> MFENITTAPADPILGLADLFRADERPGKINLGIGVYKDETGKTPVLTSVKKAEQYLLENETTKNYLGIDGIPEFGRCTQELLFGKGSALINDKRARTAQTPGGTGALRVAADFLAKNTSVKRVWVSNPSWPNHKSVFNSAGLEVREYAYYDAENHTLDFDALINSLNEAQAGDVVLFHGCCHNPTGIDPTLEQWQTLAQLSVEKGWLPLFDFAYQGFARGLEEDAEGLRAFAAMHKELIVASSYSKNFGLYNERVGACTLVAADSETVDRAFSQ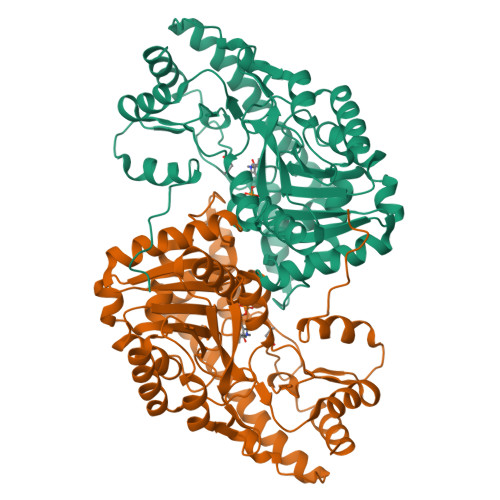MKAAIRVNYSSPPAHGASVVATILSNDALRAIWEQELTDMRQRIQRMRQLFVNTLQEKGANRDFSFTIKQNGMFFFGGLTKEQVLRLREEFGVYAVASGRLNVAGMTPDNLAPLCEAIVAVL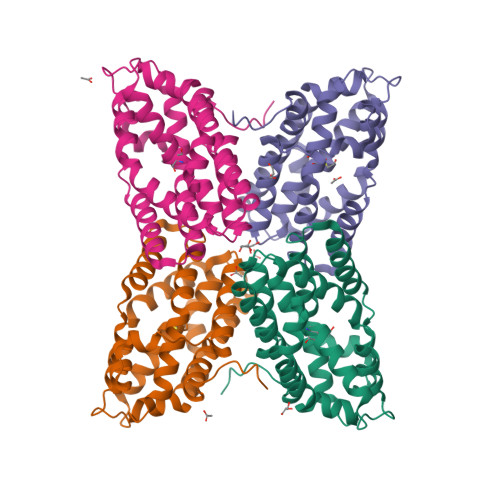>MEFSQKLYQAAKPIINDIYEDDFIQKMLLGNIQADALRHYLQADAAYLKEFTNLYALLIPKMNSMNDVKFLVEQIEFMVEGEVLAHDILAQIVGESYEEIIKTKVWPPSGDHYIKHMYFQAHSRENAIYTIAAMAPCPYIYAELAKRSQSDHKLNREKDTAKWFDFYSTEMDDIINVFESLMNKLAESMSDKELEQVKQVFLESCIHERRFFNMAMTLEQWEFGGKVND[4x]>MQDGMYQRFLRQHVHPEETGGSDRYCNLMMQRRKMTLYHCKRFNTFIHEDIWNIRSICSTTNIQCKNGKMNCHEGVVKVTDCRDTGSSRAPNCRYRAIASTRRVVIACEGNPQVPVHFDG[2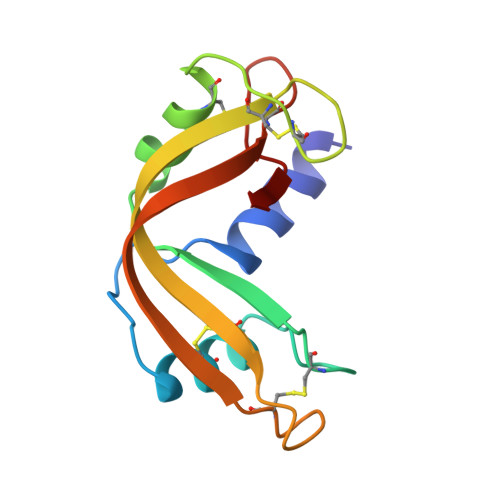x]> GSHMGEKRSIAIDSYQEDPSVVVSNFFKGVRVPKDTEFQLYKKRKQDQFVLHGENERLEYDGETDELTTKTNQYMVGLYDKQSG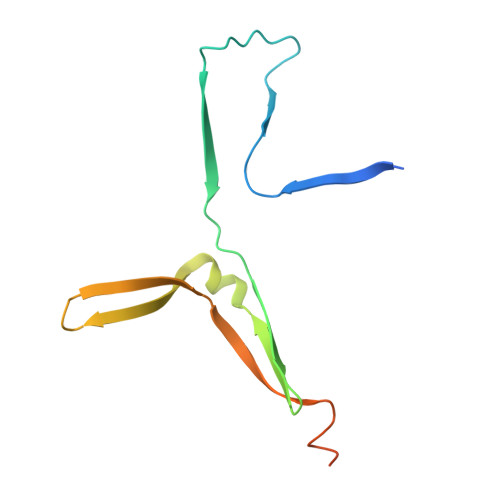KINLYRAPVVTSKIVSKFSKNLKGPEIKSKGDTRYGAM>GSIYSPHETLAEKHSEKKLMDSFSPSLSQDKMDGEFAHANIDGISIRLCLNKGICSVFYLDGDKIQSTQLSSKEYNNLLSSLPPKQFNLGKVHTITAPVSGNFKTHKPAPEVIETAINCCTSIIPNDDYFHVKDTDFN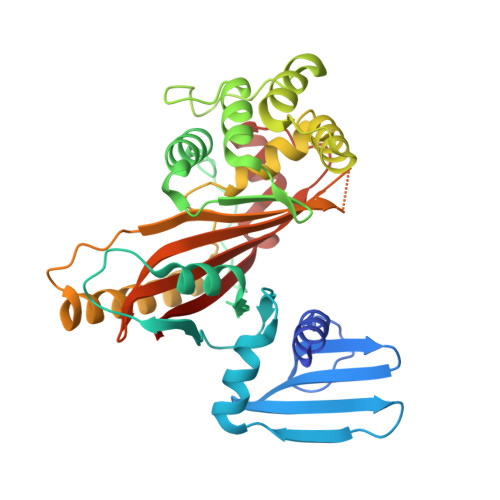SVWHDIYRDIRASDSNSTKIYFNNIEIPLKLIADLINELGINEFIDSKKELQMLSYNQVNKIINSNFPQQDLCFQTEKLLFTSLFQDPAFISALTSAFWQSLHITSSSVEHIYAQIMSENIENRLNFMPEQRVINNCGHIIKINAVVPKNDTAISASGGRAYEVSSSILPSHITCNGVGINKIETSYLVHAGTLPSSEGLRNAIPPESRQVSFAIISPDV[2x]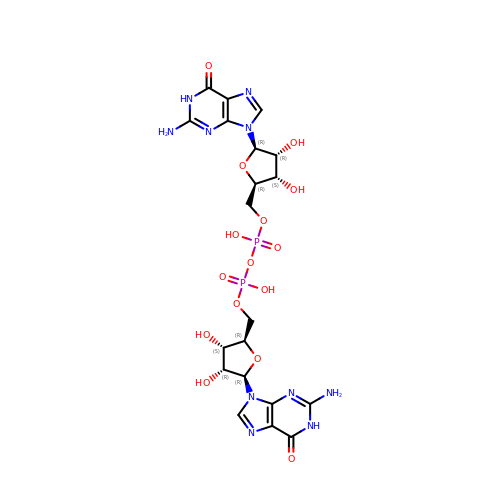[[(2~{R},3~{S},4~{R},5~{R})-5-(2-azanyl-6-oxidanylidene-1~{H}-purin-9-yl)-3,4-bis(oxidanyl)oxolan-2-yl]methoxy-oxidanyl-phosphoryl] [(2~{R},3~{S},4~{R},5~{R})-5-(2-azanyl-6-oxidanylidene-1~{H}-purin-9-yl)-3,4-bis(oxidanyl)oxolan-2-yl]methyl hydrogen phosphate | C20 H26 N10 O15 P2 | LFEYGVXBDRXHGF-MHARETSRSA-N> MKKGHHHHHHGSERTGTQPLGVQGLTEEQRMMIRELMDAQMKTFDTTFSHFKNFRLPGVLSSGCELPESLQAPSREEAAKWSQVRKDLCSLKVSLQLRGEDGSVWNYKPPADSGGKEIFSLLPHMADMSTYMFKGIISFAKVISYFRDLPIEDQISLLKGAAFELCQLRFNTVFNAETGTWECGRLSYCLEDTAGGFQQLLLEPMLKFHYMLKKLQLHEEEYVLMQAISLFSPDRPGVLQHRVVDQLQEQFAITLKSYIECNRPQPAHRFLFLKIMAMLTELRSIN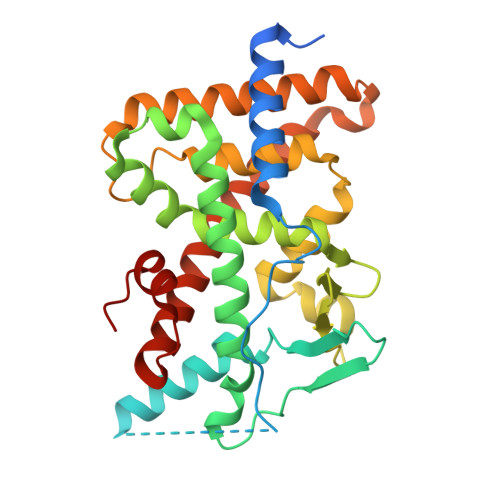AQHTQRLLRIQDIHPFATPLMQELFGITGS>[2x]ASTPQKFYLTPPQVNSILKANEYSFKVPEFDGKNVSSILGFDSNRLPANAPIEDRRSATTCLQTRGMLLGVFDGHAGCACSQAVSERLFYYIAVSLLPHETLLEIENAVESGRALLPILQWHKHPNDYFSKEASKLYFNGLRTYWQELIDLNTGESADIDVKEALINAFKRLDNDISLEAQVGDPNSFLNYLV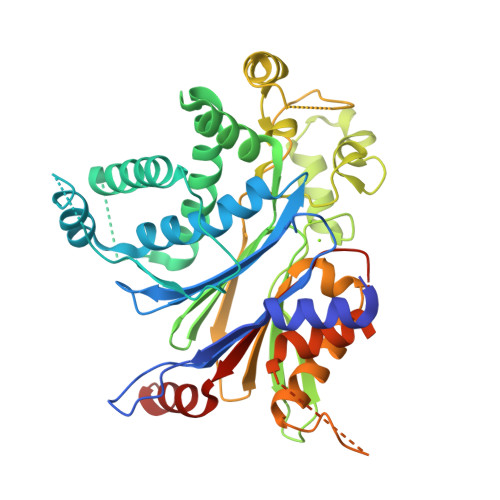LRVAFSGATACVAHVDGVDLHVANTGDSRAMLGVQEEDGSWSAVTLSNDHNAQNERELQRLKLEHPKNEAKSVVKQDRLLGLLMPFRAFGDVKFKWSIDLQKRVIESGPDQLNDNEYTKFIPPNYHTPPYLTAEPEVTYHRLRPQDKFLVLATDGLWETMHRQDVVRIVGEYLTGMHHQQPIAVGGYKVTLGQMHGLLTERRAKMSSVFEDQNAATHLIRHAVGNNEFGAVDHERLSKMLSLPEELARMYRDDITIIVVQFNSHVVGAYQNQEQ>GGCGACGAACC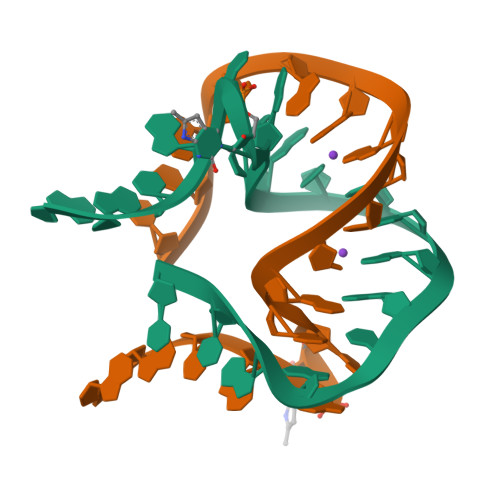GGGGAGCC[8x]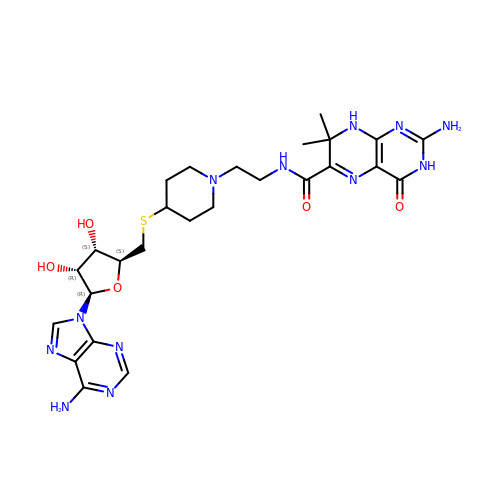5'-S-[1-(2-{[(2-amino-7,7-dimethyl-4-oxo-3,4,7,8-tetrahydropteridin-6-yl)carbonyl]amino}ethyl)piperidin-4-yl]-5'-thioadenosine | C26 H36 N12 O5 S | LXHMIPYFQUZUMS-FUKGTJLDSA-N>[2x]MEIKLQGKVSLVTGSTRGIGRAIAEKLASAGSTVIITGTSGERAKAVAEEIANKYGVKAHGVEMNLLSEESINKAFEEIYNLVDGIDILVNNAGITRDKLFLRMSLLDW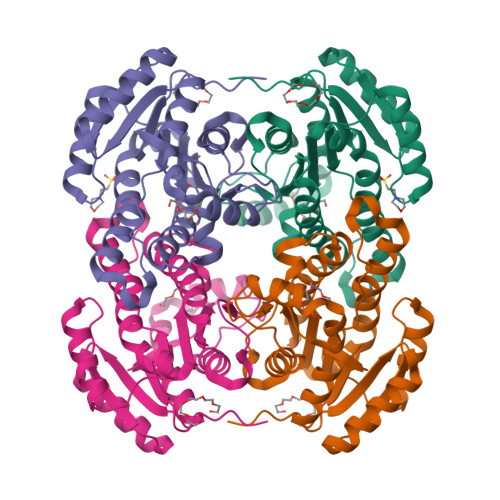EEVLKVNLTGTFLVTQNSLRKMIKQRWGRIVNISSVVGFTGNVGQVNYSTTKAGLIGFTKSLAKELAPRNVLVNAVAPGFIETDMTAVLSEEIKQKYKEQIPLGRFGSPEEVANVVLFLCSELASYITGEVIHVNGGMF>MRCFERYRVHLNRLSLSNAVMRMVSGYAPSVVGAMGWSIFSSGPAAAQSAGGGTDPATMVNNICTFILGPFGQS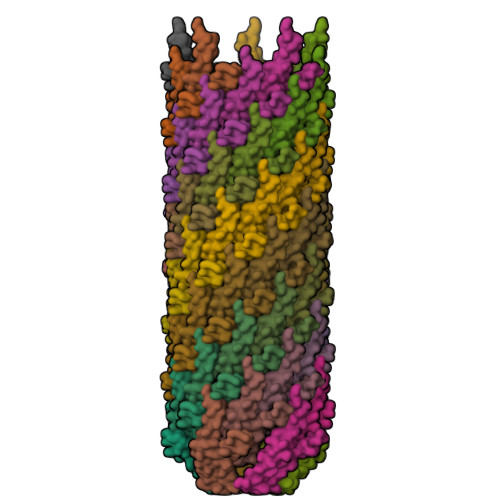LAVLGIVAIGISWMFGRASLGLVAGVVGGIVIMFGASFLGKTLTGGG[70x]2-chloro-5-[(1S)-1-hydroxy-3-oxo-2H-isoindol-1-yl]benzenesulfonamide | C14 H11 Cl N2 O4 S | 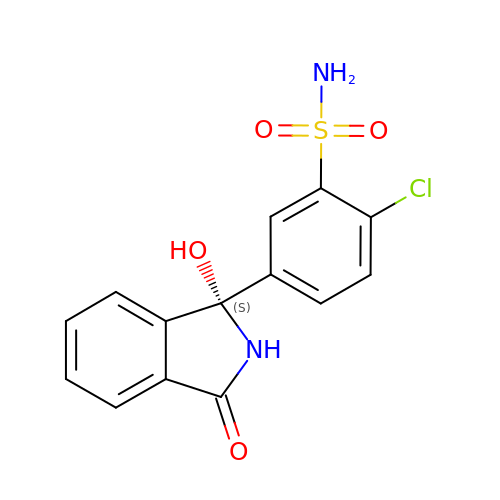JIVPVXMEBJLZRO-AWEZNQCLSA-N>CSTQLDIVIVLDGSNSIYPWESV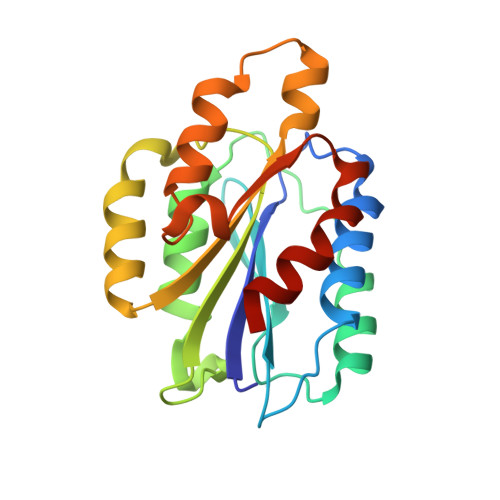IAFLNDLLKRMDIGPKQTQVGIVQYGENVTHEFNLNKYSSTEEVLVAANKIGRQGGLQTMTALGIDTARKEAFTEARGARRGVKKVMVIVTDGESHDNYRLKQVIQDCEDENIQRFSIAILGHYNRGNLSTEKFVEEIKSIASEPTEKHFFNVSDELALVTIVKALGERIFALEA[2x]> TCSQPNNFPAEIPLYKQSFKNWAGDIKVDDVWTCAPRSADEVVKVANWAKDNGYKVRARGMMHNWSPLTLAAGVSCPAVVLLDTTRYLTAMSIDASGPVAKVTAQAGITMEALLTGLEKAGLGVTAAPAPGDLTLGGVLAINGHGTAIPAKGERRLAGASYGSISNLVLSLTAVVYDKASGAYALRKFARNDPQIAPLLAHVGRSLIVEATLQAAPNQRLRCQSWFNIPYGEMFAAAGSGGRTFASYLDSA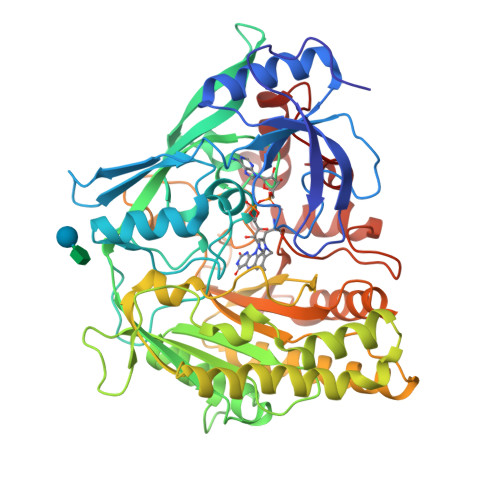GRVEAIWFPFTSNPWLKVWTVTPNKPLFSRQTDKPFNYPFSDNLPDEVTDLANKILSLGDGKLTPAFGKAQFAAASAGLVATASWDLWGWSKNLLLYVKPTTLRVTANGYAVLTRRENVQRVLNEFVTFYQARVQAYQQQGRYPMNGPVEIRVTGLDDPSEAALSGGVAPALSAIRPRPDHPEWNVAVWLDILTLPGTPYANQFYREIEQWIEANFNGSYAAVRPEWSKGWGYTDQAAWADSAMLQTTIPNAFRAGQPAAANWDAAKAALAAYDPYRLFSSPLLDSLGL> MQLF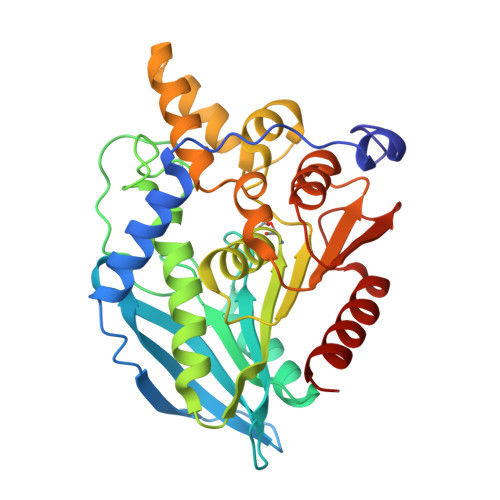DLSLEELKKYKPKKTARPDFSDFWKKSLEELRQVEAEPTLESYDYPVKGVKVYRLTYQSFGHSKIEGFYAVPDQTGPHPALVRFHGYNASYDGGIHDIVNWALHGYATFGMLVRGQGGSEDTSVTPGGHALGWMTKGILSKDTYYYRGVYLDAVRALEVIQSFPEVDEHRIGVIGGXQGGALAIAAAALSDIPKVVVADYPYLSNFERAVDVALEQPYLEINSYFRRNSDPKVEEKAFETLSYFDLINLAGWVKQPTLMAIGLIDKITPPSTVFAAYNHLETDKDLKVYRYFGHEFIPAFQTEKLSFLQKHLLLST4-(trifluoromethoxy)benzoic acid | C8 H5 F3 O3 | 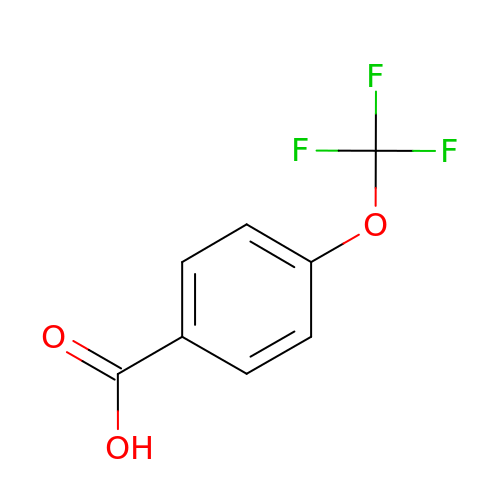RATSANVPHHXDCT-UHFFFAOYSA-N> GSSHHHHHHSSGRENLYFQGHMNGDQNSDVYAQEKQDFVQHFSQIVRVLTEDEMGHPEIGDAIARLKEVLEYNAIGGKYNRGLTVVVAFRELVEPRKQDADSLQRAWTVGWCVELLQAFFLVADDIMDSSLTRRGQICWYQKPGVGLDAINDANLLEACIYRLLKLYCREQPYYLNLIELFLQSSYQTEIGQTLDLLTAPQGNVDLVRFTEKRYKSIVKYKTAFYSFYLPIAAAMYMAGIDGEKEHA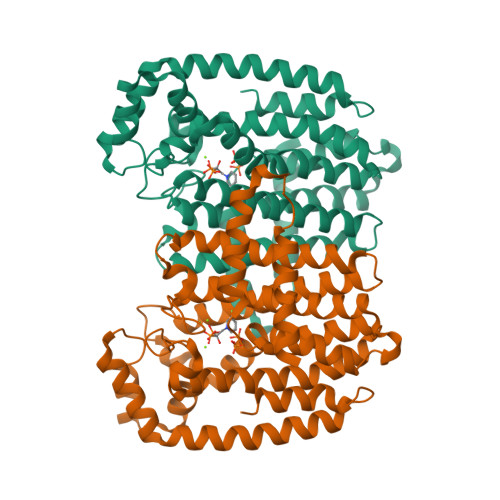NAKKILLEMGEFFQIQDDYLDLFGDPSVTGKIGTDIQDNKCSWLVVQCLQRATPEQYQILKENYGQKEAEKVARVKALYEELDLPAVFLQYEEDSYSHIMALIEQYAAPLPPAVFLGLARKIYKRRK> GSMGGPQYGIAREDVVLNRILGEGFFGEVYEGVYTNHKGEKINVAVKTCKKDCTLDNKEKFMSEAVIMKNLDHPHIVKLIGIIEEEPTWIIMELYPYGELGHYLERNKNSLKVLTLVLYSLQICKAMAYLESINCVHRDIAVRNILVASPECVKLGDFGLSR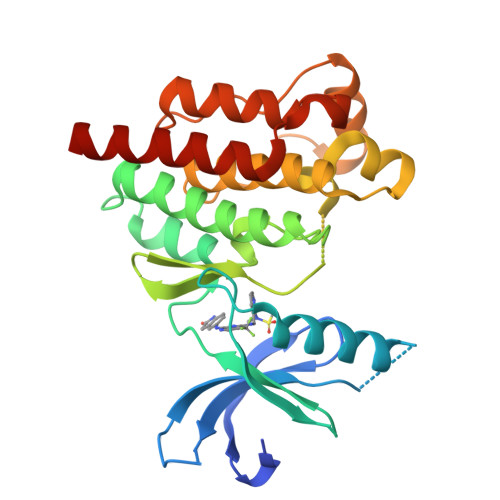YIEDEDYYKASVTRLPIKWMSPESINFRRFTTASDVWMFAVCMWEILSFGKQPFFWLENKDVIGVLEKGDRLPKPDLCPPVLYTLMTRCWDYDPSDRPRFTELVCSLSDVYQMEKDIAME6-azanyl-11-methyl-2-oxidanylidene-N-[(1S)-1-pyridin-3-ylethyl]-1,7,9-triazatricyclo[8.4.0.0^{3,8}]tetradeca-3,5,7,9,11,13-hexaene-5-carboxamide | C20 H18 N6 O2 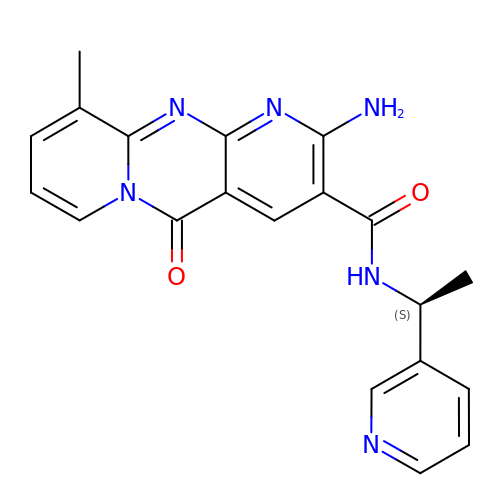| FHRKZGQIKPGLAU-LBPRGKRZSA-N Src homology 3 (SH3) domain is one of the earliest discovered and widely studied PPI modules, which can recognize a diverse array of the proline-rich motifs (PRMs). Interestingly, although varying in amino acid sequences, the SH3 domains have a conserved architecture containing five antiparallel β-strands (β1–β5) and three defined loops of RT-loop, n-Src-loop, and Distal-loop, as well as a short helix termed as 310, which form a highly conserved hydrophobic groove to recognize PRMs. ASAP1 was reported to play essential roles in both membrane trafficking (e.g., Rab8/11-coated vesicles) and actin cytoskeleton remodeling, which are highly associated with the MyoVa’s functions. Previously, we identified MICAL1, an F-actin disassembly factor, as the binding partner of Myosin Va (MyoVa) by using the globular tail domain (GTD) of MyoVa as the bait in the pulldown experiment coupled with mass spectrum analysis.

Importantly, compared with the typical SH3/PRM interactions with ~20–200 μM binding affinity, the isothermal titration calorimetry (ITC)-based analyses indicate that the interaction between ASAP1-SH3 and MICAL1-PRM has a relatively high affinity of ~1 μM. To unveil the molecular basis of such a high-affinity interaction between ASAP1 and MICAL1, using a shorter boundary (828–836) of MICAL1-PRM, we determined the crystal structure of ASAP1-SH3 and MICAL1-PRM complex at an atomic resolution of 1.17 Å with high quality. In the complex structure, ASAP1-SH3 adopts a typical SH3 fold to interact with the two crucial prolines of the PxxP core in MICAL1-PRM. In addition to the proline binding, the positively charged residue R835 (position 5) at the C-terminus of MICAL1-PRM packs with the negatively charged patch on ASAP1-SH3, indicating that MICAL1-PRM belongs to the class-II PRM. In the SEM5-SH3 structure, an aromatic residue F165 is located at the center of the hydrophobic pocket and provides hydrophobic contact with a valine (V4) in Sos-PRM, whereas in ASAP1-SH3, this position is replaced by a cysteine, C1096, which has a short sidechain and thereby unlikely contacts with a short-sidechain residue in position 2 of PRMs (e.g., V4 in Sos-PRM). Instead, such a phenylalanine-to-cystine replacement allows the long sidechain of K832 in MICAL1-PRM to fit into this pocket of ASAP1-SH3. In addition, the positively charged tip of the sidechain of K832 is fixed by the interaction with negatively charged D1099 in ASAP1-SH3, corresponding to a glutamine residue (Q168) in SEM5-SH3. Either mutation C1096F or D1099K in ASAP1-SH3 dramatically decreases the affinity for MICAL1-PRM binding to a level comparable to those of the typical SH3/PRM interactions. In contrast to the K832E mutant that completely loses the binding to ASAP1-SH3, the K832R mutation mildly enhances the ASAP1/MICAL1 interaction, confirming the requirement of the positively charged residue for the high-affinity recognition.

> GPGSEFVRRVKTIYDCQADNDDELTFIEGEVIIVTGEEDQEWWIGHIEGQPERKGVFPVSFVHILSD;> GPGSEPPPKPPRS TRICARBALLYLIC ACID | C6 H8 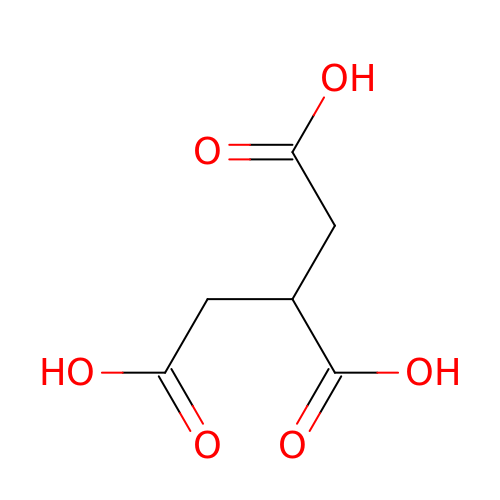O6 | KQTIIICEAUMSDG-UHFFFAOYSA-N> MKQILDSARNYLKNNSRIKTASLISLELPGSTGTSTAFIYLTDYFRDVIYNGILYQAGKVKSISPHKQNRDLSIGSLSFTITGTAQDEVLKLVQNGVSFLDRTVSIHQAIITEDGSILPVDPDTNGPLLYFRGRITGGGIKDNISTSGVGTSTITWNCSNQFYDFDRVNGRYTDDASHRGLEVVAGQLLPSNGAKRLEYQEDY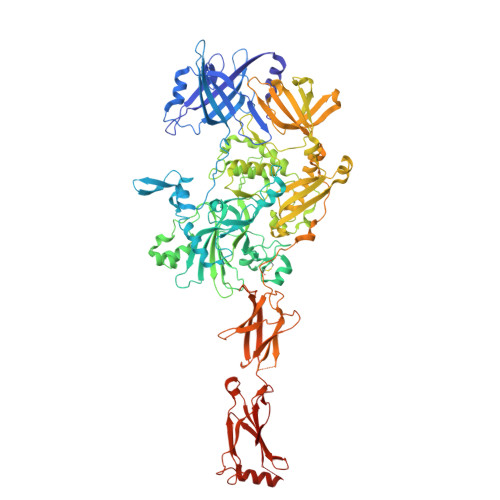GFFHANKSISILAKYQVQEERYKLKSKKKLFGLSRSYSLKKYYETVTKEVDIDFNLAAKYIPVVYGVQKIPGIPIFADTELHNPNIVYVVYAFAEGEIDGFLDFSFGDNPMICVDANDSSARTCFGTKKIVGDTMQRIASGISSSSPSVHGQEYRYNDGNGDIRIWTYHGKSNQTASDVLVNIARNRGFYLQNMNGNGPEYWDARYKLLDTAYAVVRFTINENRTEIPEVSAEIQGKKVKVYHSDGRVTANSTSLNGIWQTLDYLTSDRYGANITIDQFPLQQLIQEAAILDIIDESYQVSWQPYWRYVGWTNPLAENRQIVQMNTILDTSESVFKNVQGLLESYGGAINNLSGQYRVTVEKYSNTPLEINFLDTYGDLELSDTTGRNKFNSVQASIVDPALSWKTNSITFYNSNYKEQDKNLDKKLQLSFANITNYYTARSFADRELKKSRYSRTLSFSLPYQFIGIEPNDAIAFTYDRYGWDRKYFLVDEVENSREGKINVTLQEYGEDVFINSGQVDNSGNDIPDISNNVLPPRDFKYTPTPGGLVGSIGKNGELSWLPSLTNNVVYYSIVHSGHAEPYIVQQLETNPNERMIQEIIGEPAGLAIFEIRAVDINGRRSSPVTLSIELNSAKNLSVVSNFRVTNTASGDVTEFVGPDVKLAWDRIPEEDIIESIFYTLEIHDPQNRMLRSVRIENQYTYDYLLTYNKADFALQNSDALGINRKLYFRIRAEGDDGEQSVEWASI>MVLDIQLFRDETGANIIRESQRRRFADPDIVDAIIEADKKWRRTQFLTEASKKLINICSKAVGAKKKAKEADGDTSEIPPQVKEAYENGTLKGEQVEQLCVLQLKQLSKDLSDQVAGLAKEAQQLEEERDKLMLNVGNILHESVPIAQDEETGNTVVRTFGNTTKRAKLNHVSIMERLGMMDTSKAVTSMAGGRSYVLKGGLVQLQVALVSYSLDFLVKRGYTPFYPPFFLNRDVMGEVAQLSQFDEELYQVSGDGDKKYLIATSEMPIAAYHRGRWFTELKEPLKYAGMSTCFRKEAGAHGRDTLGIFRVHQFDKIEQFVVCS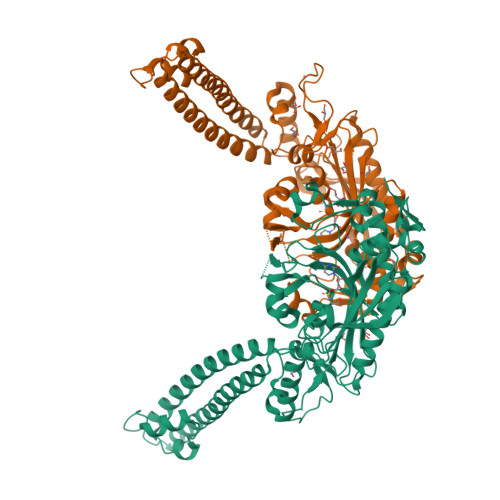PRQEESWRHLEDMITTSEEFNKSLGLPYRVVNICSGALNNAAAKKYDLEAWFPASGAFRELVSCSNCTDYQSQSVNCRYGPNLRGTAAQNVKEYCHMLNGTLCAITRTMCCICENYQTEEGVVIPDVLRPYMMGIEMIRFENNAQAEGTTPDKGE[2x]α-Methylacyl-CoA racemase in M. tuberculosis (MCR) has an essential role in fatty acid metabolism and cholesterol utilization, contributing to the bacterium’s survival and persistence. It catalyses the racemization of α-methyl-branched fatty acyl-CoAs, converting the (2S)-epimer to a near racemic mixture of the (2R)- and (2S)-epimers. The enzyme enables the conversion of α-methyl-branched fatty acids derived from cholesterol metabolism into forms that can be utilized by M. tuberculosis for growth and persistence within the host, a key component of M. tuberculosis pathogenesis. Within each active site, the large domain contributes the catalytic residues H126 (part of α-helix 3) and D156 (part of α-helix 5), while the small domain contributes a third catalytic residue, E241 (part of α-helix 9).

Crystals of the three MCR mutants H126A, D156A and E241A were obtained using identical conditions to those used with the wild-type enzyme and diffracted to 2.45, 1.64 and 1.85 Å resolutions, respectively. The overall structures for these single mutants were very similar to those of the wild-type structure, with small root-mean-squared deviation (RMSD) differences of 0.38, 0.37 and 0.38 Å for 693 Cα atoms of the H126A, D156A and E241A mutant structures being observed, respectively. The three mutants collectively had fewer hydrogen bond interactions; within the H126A, D156A and E241A mutants, 3, 5 and 5 interactions were observed, respectively. The active site of the D156A mutant has the fewest structural changes, as the H126-and-D241 dyad is retained along with the associated hydrogen bonding interactions. Within the wild-type, the D156 side-chain is hydrogen-bonded to a PEG molecule and a water molecule (which form part of a network which terminates with Y130) and a peripheral N152 residue. Consequently, as this D156 side-chain is mutated to Ala, these interactions are lost. Interestingly, the orientation peripheral N152 residue is unaffected and can form a hydrogen bond with part of the PEG molecule compared to the wild-type and the two other mutants. The rate-against-amount of enzyme plots show the expected enzyme-dependent increase in rate, while the specific activities calculated for wild-type, H126A, D156A and E241A were 46.4, 3.2, 18.5 and 12.2 µmol.min−1.mg−1. No significant change outside the enzymatic active site was observed in the three mutants, establishing that the diminution of catalytic activity is mainly attributable to disruption of the catalytic apparatus involving key hydrogen bonding and water-mediated interactions.

>MMAGPLSGLRVVELAGIGPGPHAAMILGDLGADVVRIDRPSSVDGISRDAMLRNRRIVTADLKSDQGLELALKLIAKADVLIEGYRPGVTERLGLGPEECAKVNDRLIYARMTGWGQTGPRSQQAGHDINYISLNGILHAIGRGDERPVPPLNLVGAFGGGSMFLLVGILAALWERQSSGKGQVVDAAMVDGSSVLIQMMWAMRATGMWTDTRGANMLDGGAPYYDTYECADGRYVAVGAIEPQFYAAMLAGLGLDAAELPPQNDRARWPELRALLTEAFASHDRDHWGAVFANSDACVTPVLAFGEVHNEPHIIERNTFYEANGGWQPMPAPRFSRTASSQPRPPAATIDIEAVLTDWDGGSGC[2x]>GSMDFPQHSQHVLEQLNQQRQLGLLCDCTFVVDGVHFKAHKAVLAACSEYFKMLFVDQKDVVHLDISNAAGLGQVLEFMYTAKLSLS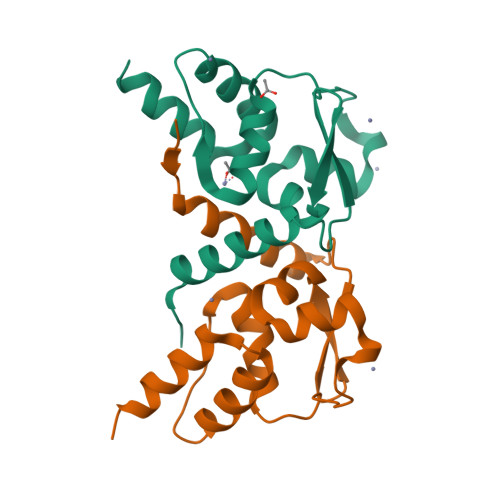PENVDDVLAVATFLQMQDIITACHALKSLA[2x]>[2x]MEKQQDLPFPYEFRELNPEEDKLVKANLGAFPTTYVKLGPKGYMVYRPYLKDAANIYNMPLRPTDVFVASYQRSGTTMTQELVWLIENDLNFEAAKTYMSLRYIYLDGFMIYDPEKQEEYNDILPNPENLDMERYLGLLEYSSRPGSSLLAAVPPTEKRFVKTHLPLSLMPPNMLDTVKMVYLARDPRDVAVSSFHHARLLYLLNKQSNFKDFWEMFHRGLYTL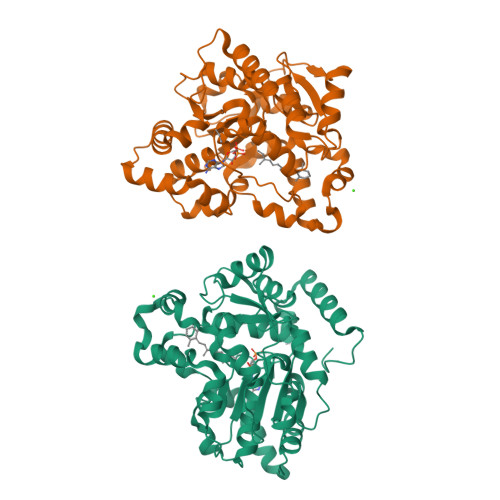TPYFEHVKEAWAKRHDPNMLFLFYEDYLKDLPGSIARIADFLGKKLSEEQIQRLSEHLNFEKFKNNGAVNMEDYREIGILADGEHFIRKGKAGCWRDYFDEEMTKQAEKWIKDNLKDTDLRYPNMEL> MSELEKAVVALIDVFHQYSGREGDKHKLKKSE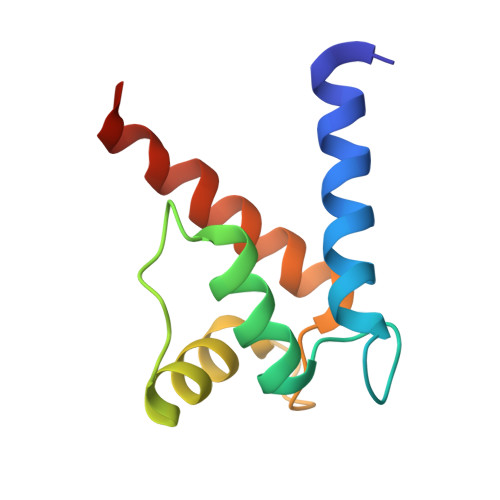LKELINNELSHFLEEIKEQEVVDKVMETLDSNGDGECDFQEFMAFVAMITTACHEFFEHE> GSRNKHHSPKRHSQTSFPAQKSTPQSQQLTSTTPQSQQQEASERSESQQIMFLSEPFVRTALVKGSFKTIVQLPKYVDLGEWIALNVFEFFTNLNQFY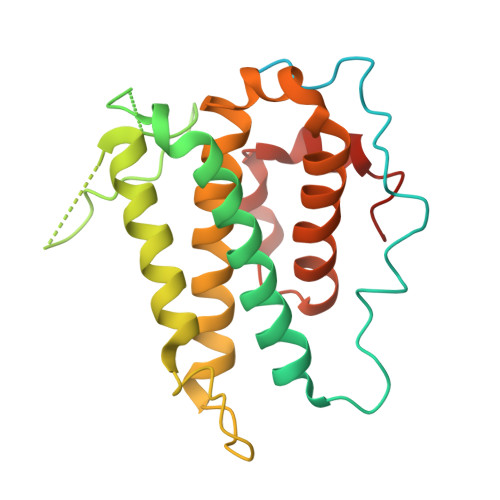GVVAEYVTPDAYPTMNAGPHTDYLWLDANNRQVSLPASQYIDLALTWINNKVNDKNLFPTKNGLPFPQQFSRDVQRIMVQMFRIFAHIYHHHFDKIVHLSLEAHWNSFFSHFISFAKEFKIIDRKEMAPLLPLIESFEKQGKIIYN>[3x]WQMKDLQAIKQEVSQAAPGSPQFMQTIRLAVQQFDPTAKDLQDLLQYLCSSLVASLH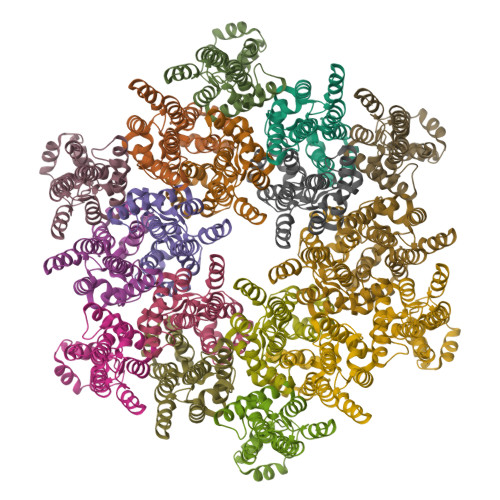HQQLDSLISEAETRGITGYNPLAGPLRVQANNPQQQGLRREYQQLWLAAFAALPGSAKDPSWASILQGLEEPYHAFVERLNIALDNGLPEGTPKDPILRSLAYSNANKECQKLLQARGHTNSPLGDMLRACQTWTP>GAAUUGCGGGAAAGGGGUCAACAGCCGUUCAGUACCAAGUCUCAGGGGAAACUUUGAGAUGGCCUUGCAAAGGGUAUGGUAAUAAG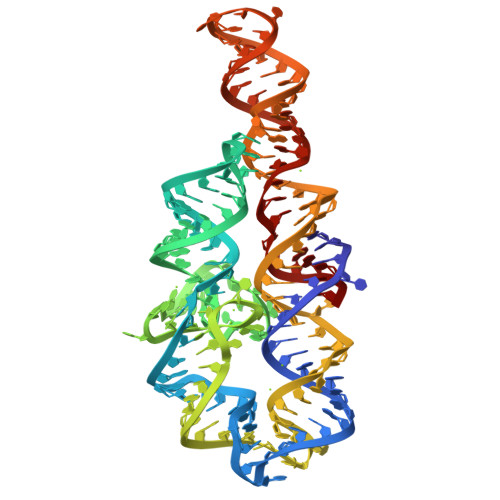CUGACGGACAUGGUCCUAACCACGCAGCCAAGUCCUAAGUCUACAGAUCUUCUGUUGAUAUGGAUGCAGUUC[2x]>[24x]MTERRVPFSLLRGPSWDPFRDWYPHSRLFDQAFGLPRLPEEWSQWLGGSSWPGYVRPLPPAAIESPAVAAPAYSRALSRQLSSGVSEIRHTADRWRVSLDVNHFAPDELTVKTKDGVVEI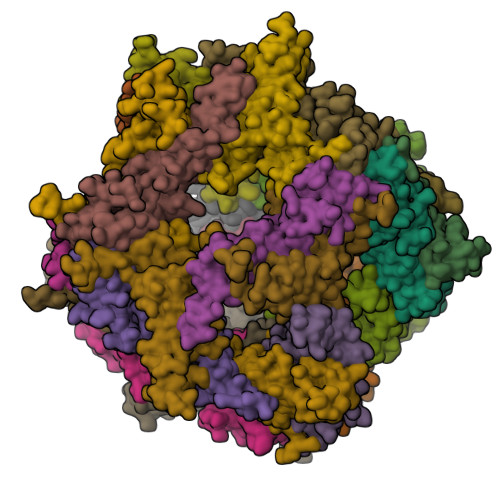TGKHEERQDEHGYISRCFTRKYTLPPGVDPTQVSSSLSPEGTLTVEAPMPKLATQSNEITIPVTFESRAQLGGPEAAKSDETAAK> CCGGACGAGGUGCGCCG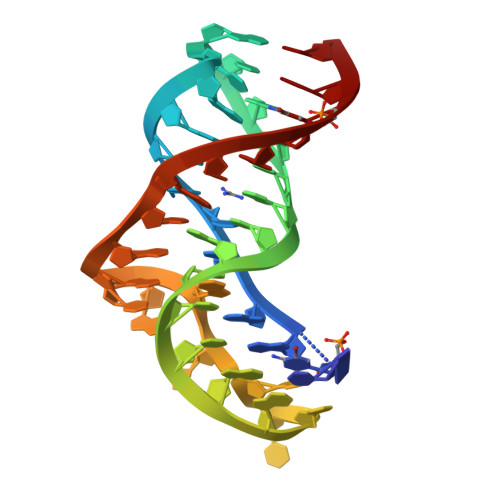UACCCGGUCACGACAAGACGGCGC N-{5-[(piperidin-1-yl)methyl]-1,3-thiazol-2-yl}acetamide | C11 H17 N3 O S | 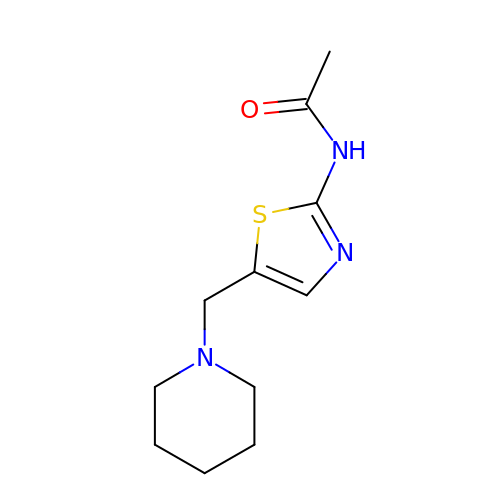WQUWVCYQJKWKDB-UHFFFAOYSA-N(3Z)-1-[(6-fluoro-4H-1,3-benzodioxin-8-yl)methyl]-4-phenyl-1H-indole-2,3-dione 3-oxime | C23 H17 F N2 O4 | 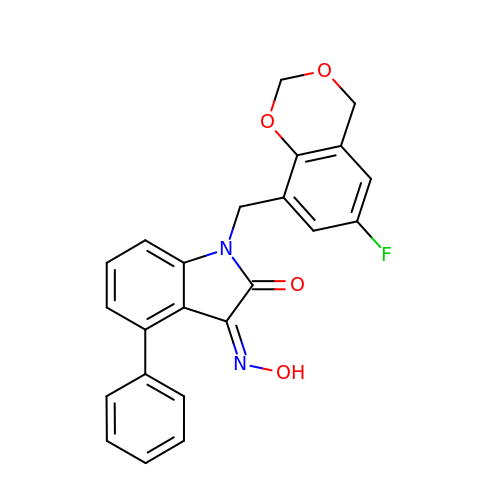SZYREAUDQRVVLV-DAFNUICNSA-N>GAMAEMDPVAEFPQPPGAARWAEVMARFAARLGAQGRRVVLVTSGGTKVPLEARPVRFLDNFSSGRRGATSAEAFLAAGYGVLFLYRARSAFPYAHRFPPQTWLSALRPSGPALSGLLSLEAEENALPGFAEALRSYQEAAAAGTFLVVEFTTL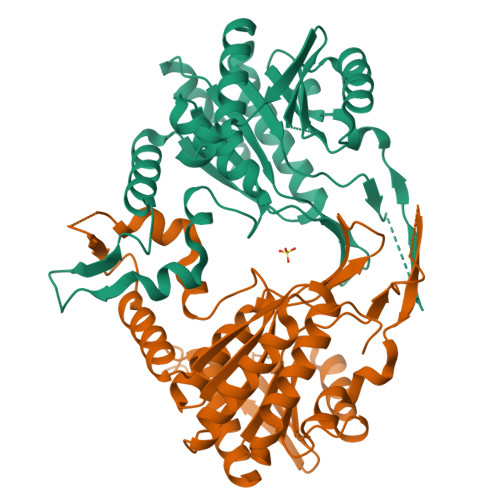ADYLHLLQAAAQALNPLGPSAMFYLAAAVSDFYVPVSEMPEHKIESSGGPLQITMKMVPKLLSPLVKDWAPKAFIISFKLETDPAIVINRARKALEIYQHQVVVANILESRQSFVLIVTKDSETKLLLSEEEIEKGVEIEEKIVDNLQSRHTAFIGDRN[2x]> MGKYLLPTAAAGLLLLAAQPAMATQGTADKDAQITQDWSVEKLYAEAQDELNSSNYTRAVKLYEILESRFPTSRHARQSQLDTAYAYYKDDEKDKALAAIERFRRLHPQHPNMDYALYLRGLVLFNEDQSFLNKLASQDWSDRDPKANREAYQAFAELVQRFPNSKYAADATARMVKLVDALGGNEMSVARYYMKRGAYIAAANRAKKIIGSYQNTRYVEESLAILELAYKKLDKPQLAADTRRVLETNFPKSPFLTHAW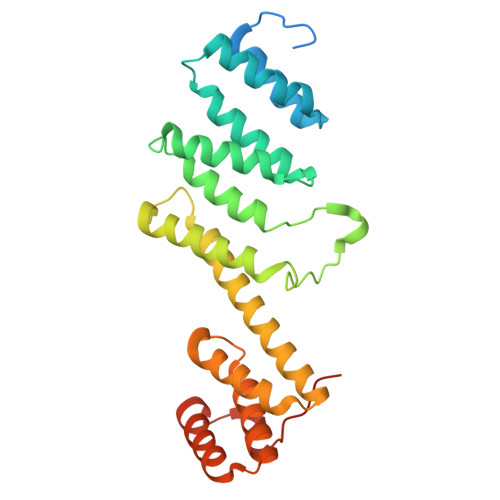QPDDMPWWRYWH> EIYCPAPPQIDNGIIQGERDHYGYRQSVTYACNKGFTMIGEHSIYCTVNNDEGEWSGPPP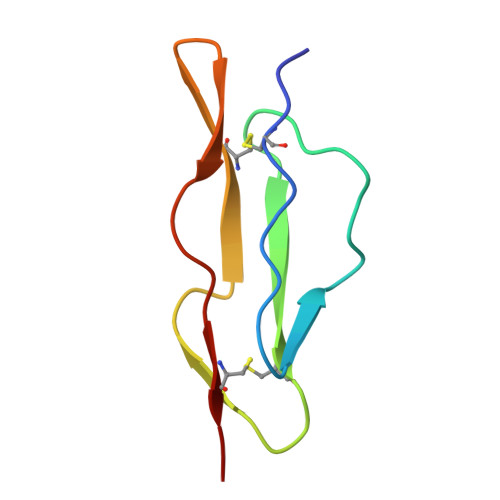ECRGC>GPGSRLDAKLVHTLPCFTFTDSAHHKAGETCAICLEDYRFGESLRLLPCQHAFHLNCIDSWLTKWGTSCPVCKHDIRTET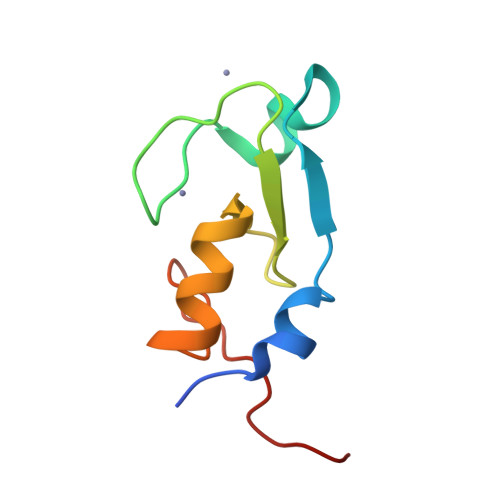MS[2x]>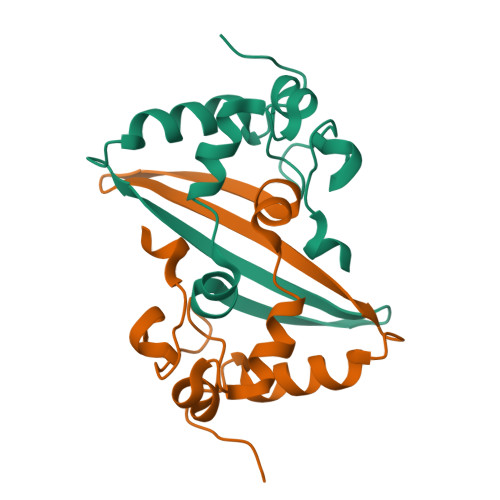RYCKRTIPPGYKVDQVFGPRTKGKEGNFGDDKMNEEGIKDGRVTAMLNLVPSSHACLFGSRVTPKLQPDGLHLKFEFTTVVPRDDPQFDNYVKICDQCVDGVGTRPKD[2x]> MM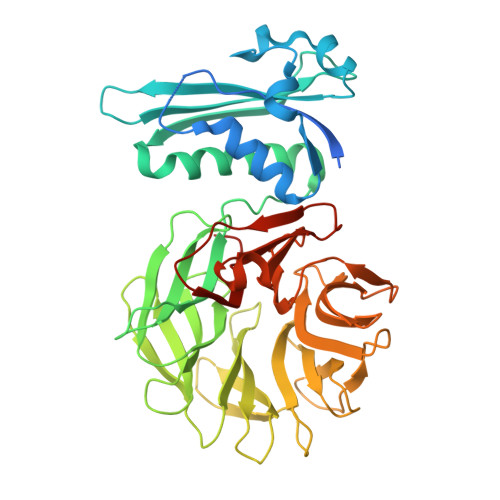KQALRVAFGFLILWASVLHAEVRIVIDSGVDSGRPIGVVPFQWAGPGAAPEDIGGIVAADLRNSGKFNPLDRARLPQQPGSAQEVQPAAWSALGIDAVVVGQVTPNPDGSYNVAYQLVDTGGAPGTVLAQNSYKVNKQWLRYAGHTASDEVFEKLTGIKGAFRTRIAYVVQTNGGQFPYELRVSDYDGYNQFVVHRSPQPLMSPAWSPDGSKLAYVTFESGRSALVIQTLANGAVRQVASFPRHNGAPAFSPDGSKLAFALSKTGSLNLYVMDLASGQIRQVTDGRSNNTEPTWFPDSQNLAFTSDQAGRPQVYKVNINGGAPQRITWEGSQNQDADVSSDGKFMVMVSSNGGQQHIAKQDLATGGVQVLSSTFLDETPSLAPNGTMVIYSSSQGMGSVLNLVSTDGRFKARLPATDGQVKFPAWSPYLLEHHHHHH>[2x]MGVPAKKKQQQGERSRESILDATERLMATKGYAATSISDIRDACGLAP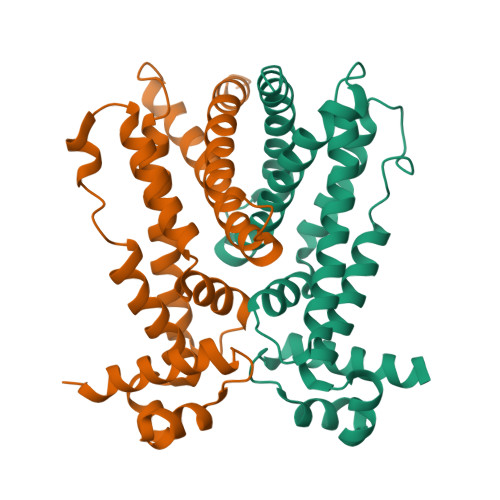SSIYWHFGSKEGVLAAMMERGAQRFFAAIPTWDEAHGPVEQRSERQLTELVSLQSQHPDFLRLFYLLSMERSQDPAVAAVVRRVRNTAIARFRDSITHLLPSDIPPGKADLVVAELTAFAVALSDGVYFAGHLEPDTTDVERMYRRLRQALEALIPVLLEETHHHHHH>[4x]MSSLDNAPLLELDVQEWVNHEGLSNEDLRGKVVVVEVFQMLCPGCVNHGVP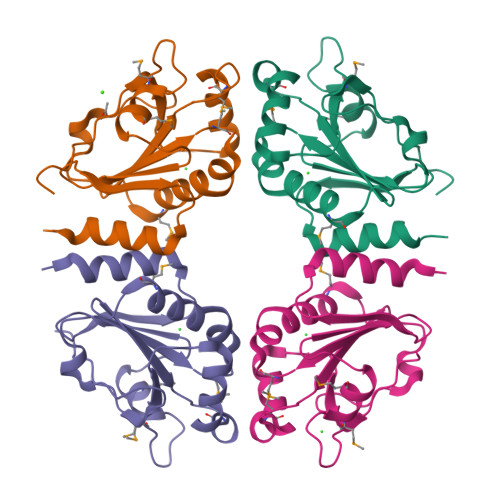QAQKIHRMIDESQVQVIGLHSVFEHHDVMTPEALKVFIDEFGIKFPVAVDMPREGQRIPSTMKKYRLEGTPSIILADRKGRIRQVQFGQVDDFVLGLLLGSLLSETDET(6R)-1-[3,5-bis(fluoranyl)-4-[2-fluoranyl-5-(hydroxymethyl)phenyl]phenyl]-6-propan-2-yl-6,7-dihydro-5H-benzotriazol-4-one | C22 H20 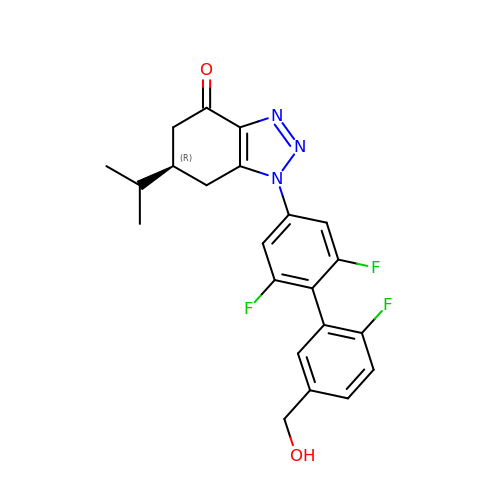F3 N3 O2 | PDEIRWICIYOXPB-CYBMUJFWSA-N>NNNGACUUAAGUCGG[2x]

Nonenzymatic template-directed RNA copying requires catalysis by divalent metal ions. The primer extension reaction involves the attack of the primer 3′-hydroxyl on the adjacent phosphate of a 5′-5′-imidazolium-bridged dinucleotide substrate. To explore the coordination of the catalytic metal ion with the imidazolium-bridged dinucleotide substrate, we examined catalysis by oxophilic and thiophilic metal ions with both diastereomers of phosphorothioate-modified substrates. High-resolution X-ray crystal structures of the products of primer extension with phosphorothioate substrates reveal the absolute stereochemistry of this interaction and indicate that catalysis by Mg2+ involves inner-sphere coordination with the nonbridging phosphate oxygen in the pro-SP position, while thiophilic cadmium ions interact with sulfur in the same position, as in one of the two phosphorothioate substrates.

The structures consistently displayed RP products at both the +1 and +2 positions, regardless of whether D1 or D2 was used as a substrate, further supporting the stereospecific coordination of Mg2+ with the pro-SP oxygen. Although we used the two different diastereomeric *psG monomers, they ultimately result in the same (R, S)-Gps*psG substrate due to the inversion of chirality at one phosphorus center during the formation of the bridged dinucleotide. The resulting primer extension products were crystallized directly without further purification, and we were able to determine the structures of both product duplexes. Mg2+ consistently leads to RP products, regardless of the stereochemistry of the substrate monomer. Given the oxophilic nature of Mg2+ ions, the lower oxygen content (pro-SP) plays a critical role in Mg2+ catalysis.> MNLEVLCGRINVENGLSLGEPGLYDQIYDRPGLPDLDVTVDATGVTVDIGAVPDSASQLGSSINAGLITIQLSEAYKINHDFTFSGLSKTTDRRLSEVFPITHDGSDGMTPDVIHTRLDGTIVVVEFTTTRSHNIGGLEAAYRTKIEKYRDPISRRVDIMENPRVFFGVIVVSSGGVLSNMPLTQDEAEELMYRFCIANEIYTKARSMDADIELQKSEEELEAISRALSFFSLFEPNIERVEGTFPNSEIEMLEQFLSTPADVDFITKTLKAKEVEAYADLCDSHYLKPEKTIQERLEINRCEAIDKTQDLLAGLHARSNKQTSLNRGTVKLPPWLPKPSSESIDIKTDSGFGSLMDHGAYGELWAKCLLDVSLGNVEGVVSDPAKELDIAISDDPEKDTPKEAKITYRRFKPALSSSARQEFSLQGVEGKKWKRMAANQKKEKESHDALSPFLDVEDIGDFLTFNNLLADSRYGDESVQRAVSILLEKASAMQDTELTHALNDSFKRNLSSNVVQWSLWVSCLAQELASALKQHCRAGEFIIKKLKFWPIYVIIKPTKSSSHIFYSLGIRKADVTRRLTGRVFSETIDAGEWELTEFKSLKTCKLTNLVNLPCTMLNSIAFWREKLGVAPWLVRKPCSELREQVGLTFLISLEDKSKTEEIITLTRYTQMEGFVSPPMLPKPQKMLGKLDGPLRTKLQVYLLRKHLDCMVRIASQPFSLIPREGRVEWGGTFHAISGRSTNLENMVNSWYIGYYKNKEESTELNALGEMYKKIVEMEEDKPSSPEFLGWGDTDSPKKHEFSRSFLRAACSSLEREIAQRHGRQWKQNLEERVLREIGTKNILDLASMKATSNFSKDWELYSEVQTKEYHRSKLLEKMATLIEKGVMWYIDAVGQAWKAVLDDGCMRICLFKKNQHGGLREIYVMDANARLVQFGVETMARCVCELSPHETVANPRLKNSIIENHGLKSARSLGPGSININSSNDAKKWNQGHYTTKLALVLCWFMPAKFHRFIWAAISMFRRKKMMVDLRFLAHLSSKSESRSSDPFREAMTDAFHGNREVSWMDKGRTYIKTETGMMQGILHFTSSLLHSCVQSFYKSYFVSKLKEGYMGESISGVVDVIEGSDDSAIMISIRPKSDMDEVRSRFFVANLLHSVKFLNPLFGIYSSEKSTVNTVYCVEYNSEFHFHRHLVRPTLRWIAASHQISETEALASRQEDYSNLLTQCLEGGASFSLTYLIQCAQLLHHYMLLGLCLHPLFGTFMGMLISDPDPALGFFLMDNPAFAGGAGFRFNLWRACKTTDLGRKYAYYFNEIQGKTKGDEDYRALDATSGGTLSHSVMVYWGDRKKYQALLNRMGLPEDWVEQIDENPGVLYRRAANKKELLLKLAEKVHSPGVTSSLSKGHVVPRVVAAGVYLLSRHCFRFSSSIHGRGSTQKASLIKLLMMSSISAMKHGGSLNPNQERMLFPQAQEYDRVCTLLEEVEHLTGKFVVRERNIVRSRIDLFQEPVDLRCKAEDLV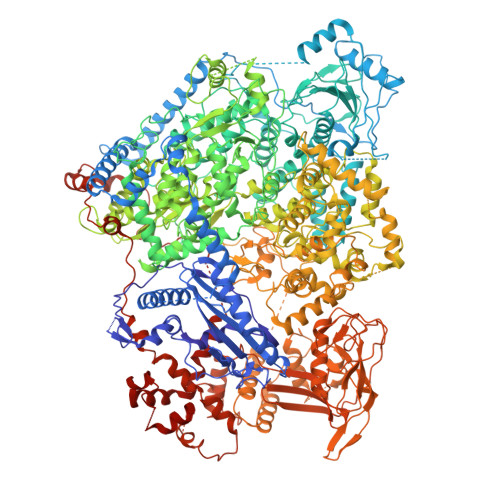SEVWFGLKRTKLGPRLLKEEWDKLRASFAWLSTDPSETLRDGPFLSHVQFRNFIAHVDAKSRSVRLLGAPVKKSGGVTTISQVVRMNFFPGFSLEAEKSLDNQERLESISILKHVLFMVLNGPYTEEYKLEMIIEAFSTLVIPQPSEVIRKSRTMTLCLLSNYLSSRGGSILDQIERAQSGTLGGFSKPQKTFIRPGGGVGYKGKGVWTGVMEDTHVQILIDGDGTSNWLEEIRLSSDARLYDVIESIRRLCDDLGINNRVASAYRGHCMVRLSGFKIKPASRTDGCPVRIMERGFRIRELQNPDEVKMRVRGDILNLSVTIQEGRVMNILSYRPRDTDISESAAAYLWSNRDLFSFGKKEPSCSWICLKTLDNWAWSHASVLLANDRKTQGIDNRAMGNIFRDCLEGSLRKQGLMRSKLTEMVEKNVVPLTTQELVDILEEDIDFSDVIAVELSEGSLDIESIFDGAPILWSAEVEEFGEGVVAVSYSSKYYHLTLMDQAAITMCAIMGKEGCRGLLTEKRCMAAIREQVRPFLIFLQIPEDSISWVSDQFCDSRGLDEESTIMWG> MCTGLALETKDGLHLFGRNMDIEYSFNQSIIFIPRNFKCVNKSNKKELTTKYAVLGMGTIFDDYPTFADGMNEKGLGCAGLNFPVYVSYSKEDIEGKTNIPVYNFLLWVLANFSSVEEVKEALKNANIVDIPISENIPNTTLHWMISDITGKSIV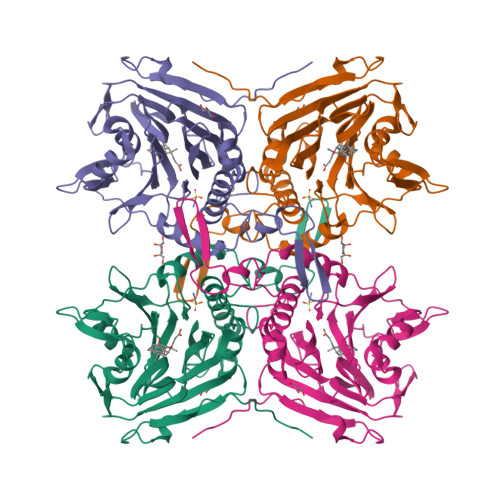VEQTKEKLNVFDNNIGVLTNSPTFDWHVANLNQYVGLRYNQVPEFKLGDQSLTALGQGTGLVGLPGDFTPASRFIRVAFLRDAMIKNDKDSIDLIEFFHILNNVAMVRGSTRTVEEKSDLTQYTSCMCLEKGIYYYNTYENNQINAIDMNKENLDGNEIKTYKYNKTLSINHVN> ARGTNVGRECCLEYFKGAIPLRKLKTWYQTS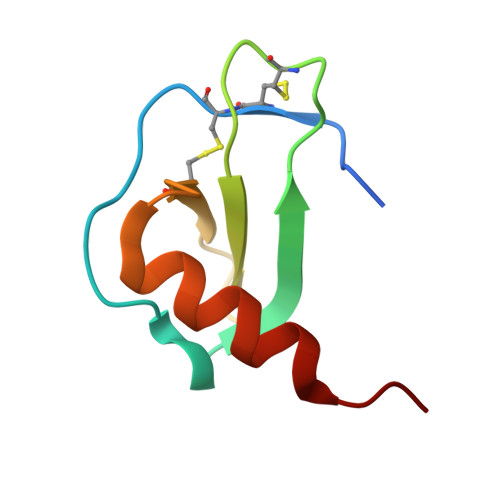EDCSRDAIVFVTVQGRAICSDPNNKRVKNAVKYLQSLERS> AFDKSAKAPVITIFDHRGCTAHKNAEYKGALTNSIDDEMCVKVQSVKIAVSEADA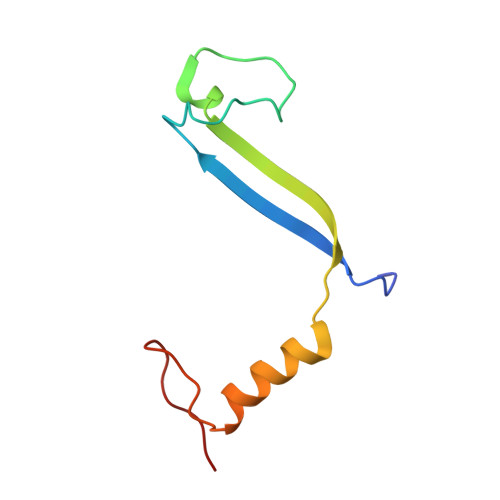AKKLQEFISYEAKGIDGAYTGRK>RSVDEGSFDITRDSKNVVESTPITIQGKEHFEGYGSVDIQKKPTDLGVSEVTRFNVGNESNGLIGALQLKNKIDFSKDFNFKVRVANNHQSNTTGADGWGFLFSKGNAEEYLTNGGILGDKGLVNSGG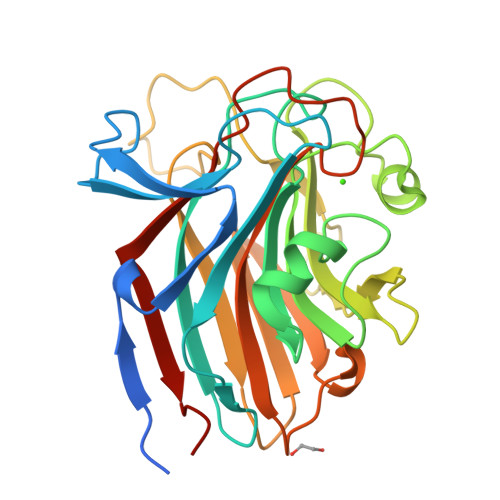FKIDTGYIYTSSMDKTEKQAGQGYRGYGAFVKNDSSGNSQMVGENIDKSKTNFLNYADNSTNTSDGKFHGQRLNDVILTYVASTGKMRAEYAGKTWETSITDLGLSKNQAYNFLITSSQRWGLNQGINANGWMRTDLKGSEFTFTPEAPKTI[4x]>[2x]KSNQENINSLKYKELIAGELMRITHKLLIQKLQQQQPANNNKQINEMDVESNELAEKKEVIIKIQEIAKDQQLYDTLSIQYQVDQKEQYYAKIAQSLEDFVSISALKMV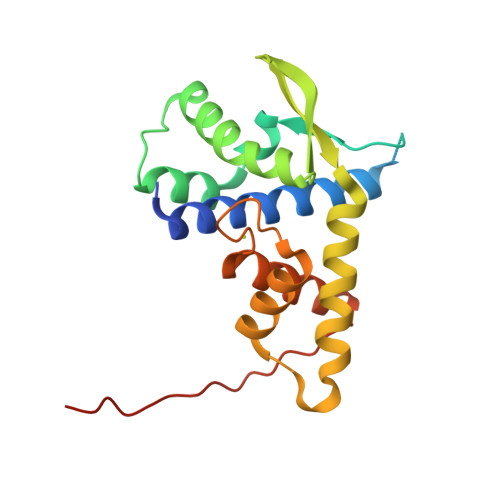SYIYPNISYQVSIGFFQNILDIATKTVKDRGALGCNYKYLKDKLTKALNLQQISYPLISESYISYLVHLFQDFNIIEIENEHKFYYKQAFQYDDS The armadillo repeat serves as a scaffold for the development of modular peptide-recognition modules. In order to develop such a system, three crystal structures of designed armadillo-repeat proteins with third-generation N-caps (YIII-type), four or five internal repeats (M-type) and second-generation C-caps (AII-type) were determined at 1.8 Å (His-YIIIM4AII), 2.0 Å (His-YIIIM5AII) and 1.95 Å (YIIIM5AII) resolution and compared with those of variants with third-generation C-caps. All constructs are full consensus designs in which the internal repeats have exactly the same sequence, and hence identical conformations of the internal repeats are expected.

The crystal structures of His-YIIIM4AII and His-YIIIM5AII were refined at 1.8 and 2.0 Å resolution, respectively. In both cases the asymmetric units contain tetramers with 222 point symmetry and very similar topologies. The quaternary structures of His-YIIIM4AII and His-YIIIM5AII are governed by calcium ions that connect neighbouring chains in a zipper-like manner and the His6 tag that binds to the supposed peptide-binding site, albeit in different orientations (see below). In contrast to this, the crystallographic tetramer of His-YIIIM5AII is less symmetric. Here, chains A/B and C/D are pairwise identical (r.m.s.d. of 0.05 Å), whereas an r.m.s.d. of 0.85 Å for the comparison between pairs (e.g. chain A with D) suggests substantial differences. Furthermore, His-YIIIM5AII chains A/B are more similar to His-YIIIM4AII (r.m.s.d. of 0.72 Å for the superposition of residues 14–210 on the equivalent residues from His-YIIIM4AII) than chains C/D (r.m.s.d. of 1.17 Å). These differences are caused by different contacts within the tetramer. The structures of His-YIIIM4AII and YIIIM5AII represent extreme cases that are most different. In His-YIIIM5AII these differences are combined into a single structure. His-YIIIM5AII chains A/B and C/D represent the conformations seen in His-YIIIM4AII (all chains) and YIIIM5AII (all chains), respectively.

>HHHHHHGSELPQMVQQLNSPDQQELQSALRKLSQIASGGNEQIQAVIDAGALPALVQLLSSPNEQILQEALWTLGNIASGGNEQIQAVIDAGALPALVQLLSSPNEQILQEALWTLGNIASGGNEQIQAVIDAGALPALVQLLSSPNEQILQEALWTLGNIASGGNEQIQAVIDAGALPALVQLLSSPNEQILQEALWTLGNIASGGNEQIQAVIDAGALPALVQLLSSPNEQILQEALWTLGNIASGGNEQKQAVKEAGALEKLEQLQSHENEKIQKEAQEALEKLQA[4x]>MGDIQVQVNIDDNGKNFDYTYTVTTESELQKVLNELMDYIKKQGAKRVRISITARSSKEAYKFLAILAKVFAELGYNDINRKMTVRFRGDDLEALEKALKEMIRQARKFAGTVTYTLDGNDLEITITG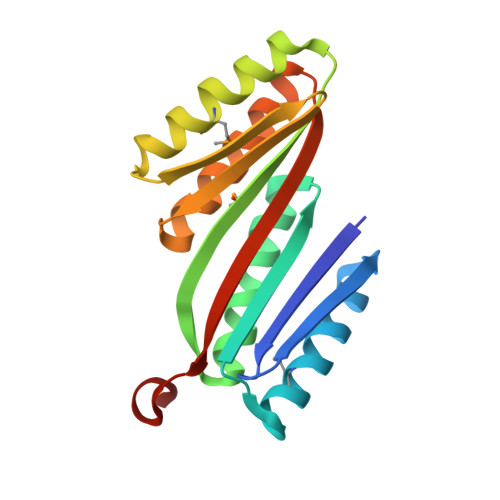VPRQVLEELAKEAERLAKEFNITITITVTVEGQLGSLEHHHHHH[4x]> GAGCAGACGTG;> ACCGCACTCA;> CAGGT;> TCTGAGTGCCGTCTGC

In this work, we exhaustively probe the ability of all 36 immobile HJ sequences to form DNA crystals in two different designed systems. Three separate self-assembling DNA crystal systems are described in this report: the “4 × 5” and “4 × 6” designs (collectively referred to as the 4 × N systems), and a third construct with a “scrambled” sequence variant of the 4 × 6 lattices. Self-assembly was mediated by three constituent oligonucleotides: (S1) containing four sequence repeats of either 5 or 6 bases; (S2) composed of 21 bases containing complementary regions to both (S1); and (S3) which forms the second junction crossover. The HJ serves as the fundamental component at the core of each unit, and the ultimate assembly of the full lattice is facilitated by the complementary 2-base sticky ends that tail each duplex.

We hypothesized that it might be possible to introduce other unique immobile sequences that could provide slight perturbations in the junction angle, to potentially reduce the strain in the original system and yield a “relaxed,” periodic lattice. The 4 × 5 system robustly crystallized with 75% of the junctions, and we obtained crystals in all but 9 of 36 sequences. Of the resulting structures, 18 exhibited P32 symmetry with average cell dimensions a = b = 68.85 Å c = 60.09 Å, with only nine retaining the original P3221 symmetry with average cell edges a = b = 68.17 Å c = 60.60 Å. Although the cell parameters between the two symmetries were virtually indistinguishable, the differences between the periodicity of the lattices is dramatic, with vastly different cavity sizes. While the highest resolution achieved for the J1 system was 3.1 Å, in roughly half of the crystals measured the resolutions were 3.05 Å or better, and as high as 2.9 Å (J6) and 2.75 Å (J19), for the P32 and P3221 symmetries, respectively. The mean angles across all junctions within the groups were 56.05° (σ = 1.63) and 56.59° (σ = 1.50) for the P32 and P3221, respectively. We hypothesize that even a small difference in junction angles could have a significant global effect on the assembly of the lattice, thereby eliminating the strain in the P3221 lattices. However, in the majority of the crystal structures reported here, the cacodylate anion indeed fits best into the electron density map of our X-ray structures, due to the presence of sodium cacodylate in the crystallization solution.> MQRRDFLKYSVALGVASALPLWSRAVFAAERPTLPIPDLLTTDARNRIQLTIGAGQSTFGGKTATTWGYNGNLLGPAVKLQRGKAVTVDIYNQLTEETTLHWHGLEVPGEVDGGPQGIIPPGGKRSVTLNVDQPAATCWFHPHQHGKTGRQVAMG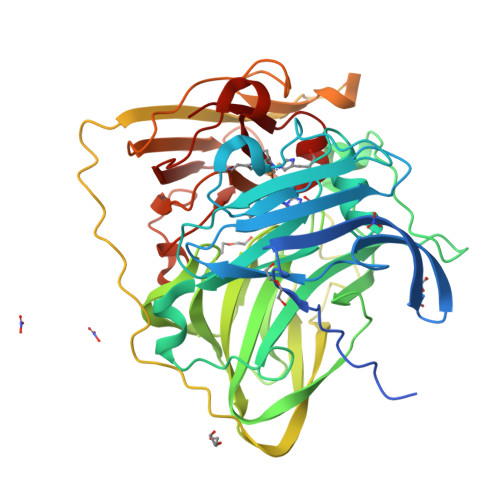LAGLVVIEDDEILKLMLPKQWGIDDVPVIVQDKKFSADGQIDYQLDVMTAAVGWFGDTLLTNGAIYPQHAAPRGWLRLRLLNGCNARSLNFATSDNRPLYVIASDGGLLPEPVKVSELPVLMGERFEVLVEVNDNKPFDLVTLPVSQMEMAIAPFDKPHPVMRIQPIAISASGALPDTLSSLPALPSLEGLTVRKLQLSMDPMLDMMGMQMLMEKYGDQAMAGMDHSQMMGHMGHGNMNHMNHGGKFDFHHANKINGQAFDMNKPMFAAAKGQYERWVISGVGDMMLHPFHIHGTQFRILSENGKPPAAHRAGWKDTVKVEGNVSEVLVKFNHDAPKEHAYMAHCHLLEHEDTGMMLGFTV>[3x]MEPHVLGAGLYWLLLPCTLLAASLLRFNALSLVYLLFLLLLPWLPGPSRHSIPGHTGRLLRALLCLSLLFLVAHLAFQICLHTVPHLDQFLGQNGSLWVKVSQHIGVTRLDLKDIFNTTRLVAPDLGVLLASSLCLGLCGRLTRKAGQSRRTQELQDDDDDDDDDDEDIDAAPAVGLKGAPALATKRRLWLASRFRVTAHWLLMTSGRTLVIVLLALAGIAHPSAFSSIYLVVFLAICTWWSCHFPLSPLGFNTLCVMVSCFGAGHLICLYCYQTPFIQDMLPPGNIWARLFGLKNFVDLPNYSSPNALVLNTKHAWPIYVSPGILLLLYYTATSLLKLHKSCPSELRKETPREDEEHELELDHLEPEPQARDATQGEMPMTTEPDLDNCTVHVLTSQSPVRQRPVRPRLAELKEMSPLHGLGHLIMDQSYVCALIAMMVWSIMYHSWLTFVLLLWACLIWTVRSRHQLAMLCSPCILLYGLTLCCLRYVWAMELPELPTTLGPVSLHQLGLEHTRYPCLDLGAMLLYLLTFWLLLRQFVKEKLLKKQKVPAALLEVTVADTEPTQTQTLLRSLGELVTGIYVKYWIYVCAGMFIVVSFAGRLVVYKIVYMFLFLLCLTLFQVYYTLWRKLLRVFWWLVVAYTMLVLIAVYTFQFQDFPTYWRNLTGFTDEQLGDLGLEQFSVSELFSSILIPGFFLLACILQLHYFHRPFMQLTDLEHVPPPGTRHPRWAHRQDAVSEAPLLEHQEEEEVFREDGQSMDGPHQATQVPEGTASKWGLVADRLLDLAASFSAVLTRIQVFVRRLLELHVFKLVALYTVWVALKEVSVMNLLLVVLWAFALPYPRFRPMASCLSTVWTCIIIVCKMLYQLKIVNPHEYSSNCTEPFPNNTNLQPLEINQSLLYRGPVDPANWFGVRKGYPNLGYIQNHLQILLLLVFEAVVYRRQEHYRRQHQQAPLPAQAVCADGTRQRLDQDLLSCLKYFINFFFYKFGLEICFLMAVNVIGQRMNFMVILHGCWLVAILTRRRREAIARLWPNYCLFLTLFLLYQYLLCLGMPPALCIDYPWRWSKAIPMNSALIKWLYLPDFFRAPNSTNLISDFLLLLCASQQWQVFSAERTEEWQRMAGINTDHLEPLRGEPNPIPNFIHCRSYLDMLKVAVFRYLFWLVLVVVFVAGATRISIFGLGYLLACFYLLLFGTTLLQKDTRAQLVLWDCLILYNVTVIISKNMLSLLSCVFVEQMQSNFCWVIQLFSLVCTVKGYYDPKEMMTRDRDCLLPVEEAGIIWDSICFFFLLLQRRIFLSHYFLHVSADLKATALQASRGFALYNAANLKSINFHRQIEEKSLAQLKRQMKRIRAKQEKYRQSQASRGQLQSKDPQDPSQEPVIHSGDYFLFESDSEEEEEALPEDPRPAAQSAFQMAYQAWVTNAQTVLRQRRERARQERAEQLASGGDLNPDVEPVDVPEDEMAGRSHMMQRVLSTMQFLWVLGQATVDGLTRWLRAFTKHHRTMSDVLCAERYLLTQELLRVGEVRRGVLDQLYVGEDEATLSGPVETRDGPSTASSGLGAEEPLSSMTDDTSSPLSTGYNTRSGSEEIVTDAGDLQAGTSLHGSQELLANARTRMRTASELLLDRRLHIPELEEAERFEAQQGRTLRLLRAGYQCVAAHSELLCYFIIILNHMV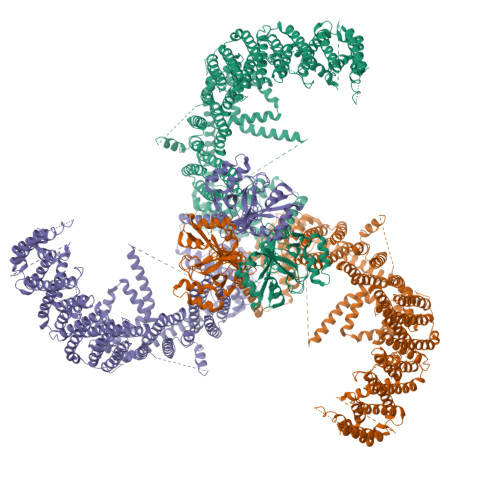TASAASLVLPVLVFLWAMLTIPRPSKRFWMTAIVFTEVMVVTKYLFQFGFFPWNSYVVLRRYENKPYFPPRILGLEKTDSYIKYDLVQLMALFFHRSQLLCYGLWDHEEDRYPKDHCRSSVKDREAKEEPEAKLESQSETGTGHPKEPVLAGTPRDHIQGKGSIRSKDVIQDPPEDLKPRHTRHISIRFRRRKETPGPKGTAVMETEHEEGEGKETTERKRPRHTQEKSKFRERMKAAGRRLQSFCVSLAQSFYQPLQRFFHDILHTKYRAATDVYALMFLADIVDIIIIIFGFWAFGKHSAATDIASSLSDDQVPQAFLFMLLVQFGTMVIDRALYLRKTVLGKLAFQVVLVVAIHIWMFFILPAVTERMFSQNAVAQLWYFVKCIYFALSAYQIRCGYPTRILGNFLTKKYNHLNLFLFQGFRLVPFLVELRAVMDWVWTDTTLSLSNWMCVEDIYANIFIIKCSRETEKKYPQPKGQKKKKIVKYGMGGLIILFLIAIIWFPLLFMSLIRSVVGVVNQPIDVTVTLKLGGYEPLFTMSAQQPSIVPFTPQAYEELSQQFDPYPLAMQFISQYSPEDIVTAQIEGSSGALWRISPPSRAQMKQELYNGTADITLRFTWNFQRDLAKGGTVEYTNEKHTLELAPNSTARRQLAQLLEGRPDQSVVIPHLFPKYIRAPNGPEANPVKQLQPDEEEDYLGVRIQLRREQVGTGASGEQAGTKASDFLEWWVIELQDCKADCNLLPMVIFSDKVSPPSLGFLAGYGIVGLYVSIVLVVGKFVRGFFSEISHSIMFEELPCVDRILKLCQDIFLVRETRELELEEELYAKLIFLYRSPETMIKWTRERE> VQQLSLFGSIGDDGYDLLISTLTTISGNPPLLYNSLCTVWKPNPSYDVENVNSRNQLVEPNRIKLSKEVPFSYLIDETMMDKPLNFRILKSFTNDKIPLNYAMTRNILHNTVPQVTNFNSTNEDQNNSKHTEDTVNESRNSDDIIDVDMDASPAPSNESCSPWSLQISDIP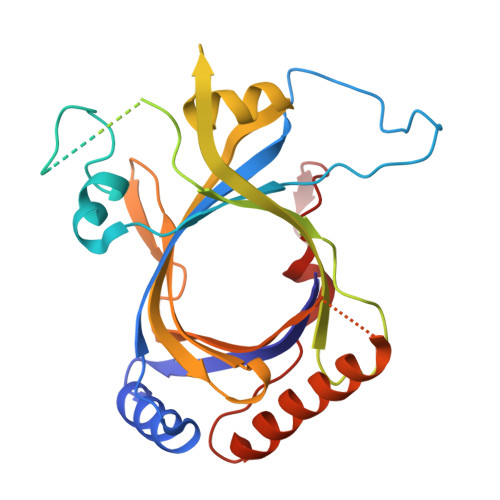AAGNNRSVSMQTIAETIILSSAGKNSSVSSLMNGLGYVFEFQYLTIGVKFFMKHGLILELQKIWQIEEAGNSQITSGGFLLKAYINVSRGTDIDRINYTETVLMNLKKELQGYIELSVPDRQSMDSRVAHGNILI>[4x]MPEVVFGSVTDLGYAAGWRLVRAMPEAMAQGVFGAGARYAARNGGPEQLRRNLARVVGKPPADVPDDLIRASLASYARYWREAFRLPAMDHGRLGEQLDVIDIDHLWSALDAGRGAVLALPHSGNWDMAGVWLVQNYGPFTTVAERLKPESLYRRFVEYRESLGFEVLPLTGGERPPFEVLAERLTDNRPICLMAERDLTRSGVQVDFFGEATRMP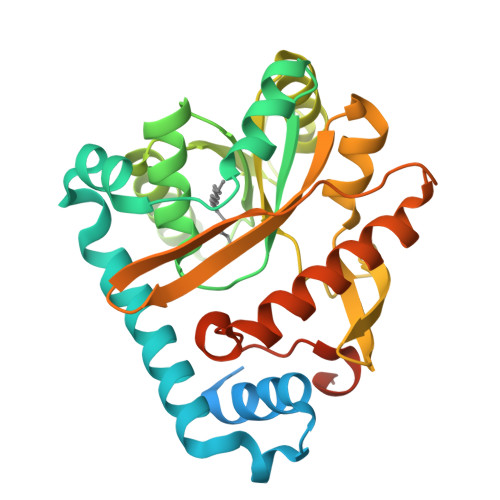AGPAKLAIETGAALFPVHCWFEGDGWGMRVYPELDTSSGDVTAITQALADRFAANIATYPADWHMLQPQWIADLSDERRARLGTSRHHHHHH>[2x]MKIRDLLKARRGPLFSFEFFPPKDPEGEEALFRTLEELKAFRPAFVSITYGAMGSTRERSVAWAQRIQSLGLNPLAHLTVAGQSRKEVAEVLHRFVESGVENLLALRGDPPRGERV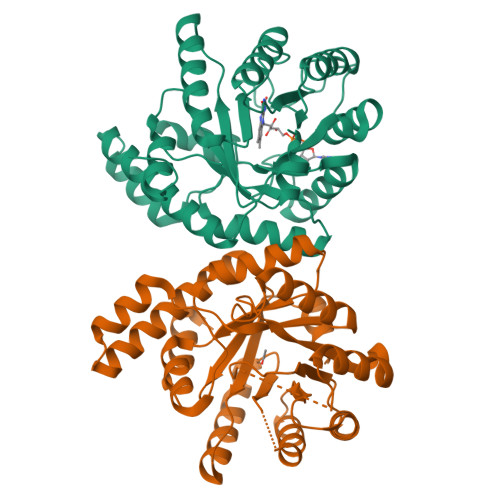FRPHPEGFRYAAELVALIRERYGDRVSVGGAAYPEGHPESESLEADLRHFKAKVEAGLDFAITQLFFNNAHYFGFLERARRAGIGIPILPGIMPVTSYRQLRRFTEVCGASIPGPLLAKLERHQDDPKAVLEIGVEHAVRQVAELLEAGVEGVHFYTLNKSPATRMVLERLGLRPASGQPAKLAAALEHHHHHH The bacteriophage ϕ29, a representative of bacteriophages with a short non-contractile tail, has an ~19 kb dsDNA genome encoding ~20 proteins. Both 5ʹ ends of the genome are covalently connected to the terminal protein gene product 3 (gp3). ϕ29 infects the Gram-positive Bacillus subtilis cells by injecting the genome–gp3 complex into the host-cell cytoplasm using a short non-contractile tail, leaving the genome emptied virion on the cell surface. Here, we report the cryo-electron microscopy (cryo-EM) structural studies of the ϕ29 prohead, the mature and the genome-emptied virions at near-atomic resolutions up to 3.2 Å. Our results show structural details of the complex capsid, the DNA packaging motor and the entire tail machinery, and provide a molecular basis for understanding the assembly, maturation and infection mechanisms of the bacteriophage ϕ29.

A dsDNA packaging machinery is assembled on the prohead by attaching a viral encoded short prohead RNA (pRNA) and the ATPase gp16 around the connector. We determined the structure of the pRNA ring at a resolution of 4.6 Å through focused classifications and refinements. Five pRNA molecules and structural features of the RNA duplexes could be clearly identified in the ring of pRNA density. An atomic model consisting of the 5ʹ 69 nts (26–94) of the pRNAs was built based on the reconstruction. Densities of the 5ʹ 25 nts (1–25) and 3ʹ 80 nts (95–174) of the pRNAs were not visible in the map, probably due to the flexibility of the corresponding nts. Our results showed that the five pRNAs assemble to form a pentameric ring structure around the narrow end of the connector. The inner diameter of the pentameric pRNA ring is ~85 Å, which is slightly larger than the narrow end of the prohead connector. However, the pRNA assembly does not have any direct close contact with the connector. Instead, the upper protrusions of the pRNA ring show extensive interactions with the E loops of the capsid through three nucleotides (U54G55A56). Based on our near-atomic resolution structures of the pRNAs, it can be confirmed that there are five pRNA molecules in the ring-shaped RNA structure.

>[5x]UCAAUGGUACGGUACUUCCAUUGUCAUGUGUAUGUUGGGGAUUAAACCCUGAUUGAGUUCAGCCCACAUACUUUGUUGAUUGGUUGUCAAUCAUGGCAAAAGUGCACGCUACUUUGAUAA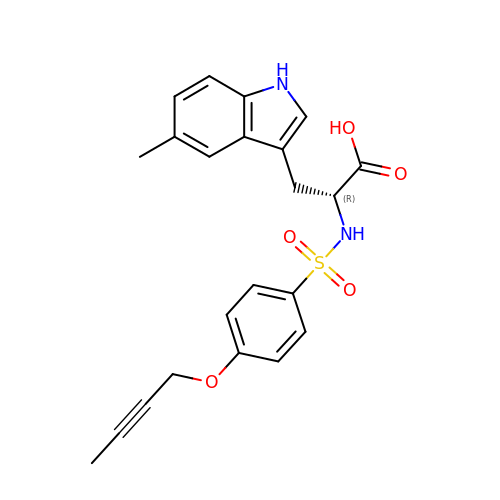N-{[4-(but-2-yn-1-yloxy)phenyl]sulfonyl}-5-methyl-D-tryptophan | C22 H22 N2 O5 S | SFVPXERGVLDWIS-OAQYLSRUSA-N> GPGSSKHLNPGLQLYRASYEKNLPKMAEALAHGADVNWANSEENKATPLIQAVLGGSLVTCEFLLQNGANVNQRDVQGRGPLHHATVLGHTGQVCLFLKRGANQHATDEEGKDPLSIAVEAANADIVTLLRLARM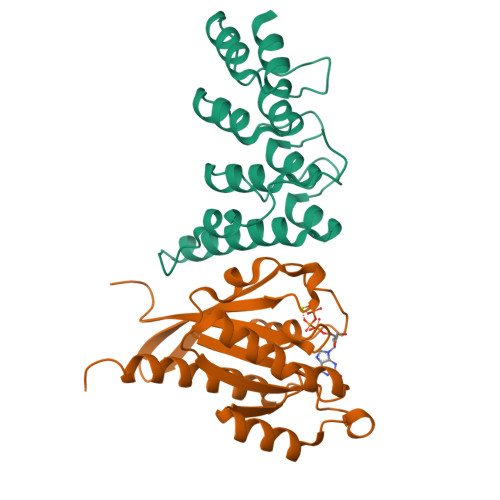NEEMRESEGLYGQPGDETYQDIFRDFSQMASNNPEKLNR;> GPGSEFMARDYDHLFKLLIIGDSGVGKSSLLLRFADNTFSGSYITTIGVDFKIRTVEINGEKVKLQIWDTAGLERFRTITSTYYRGTHGVIVVYDVTSAESFVNVKRWLHEINQNCDDVCRILVGNKNDDPERKVVETEDAYKFAGQMGIQLFETSAKENVNVEEMFNCITELVLRAKKDNLAKQQ> GPMPVFHTRTIESILEPVAQQISHLVIMHEEGEVDGKAIPDLTAPVAAVQAAVSNLVRVGKETVQTTEDQILKRDMPPAFIKVENACTKLVQAAQMLQSDP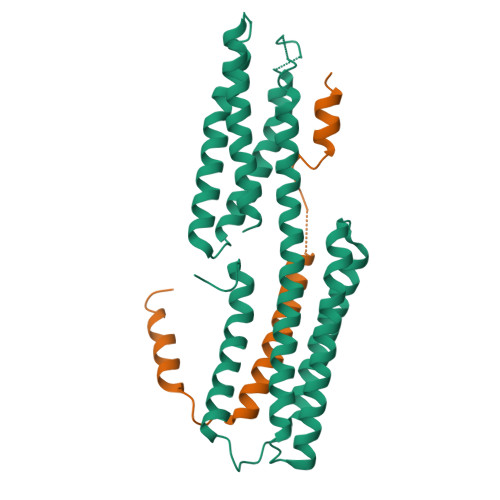YSVPARDYLIDGSRGILSGTSDLLLTFDEAEVRKIIRVCKGILEYLTVAEVVETMEDLVTYTKNLGPGMTKMAKMIDERQQELTHQEHRVMLVNSMNTVKELLPVLISAMKIFVTTKNSKNQGIEEALKNRNFTVEKMSAEINEIIRVLQL;> GPGELAYALNNFDKQIIVDPLSFSEERFRPSLEERLESIISGAALMADSSCTRDDRRERIVAECNAVRQALQDLLSEYMGNAGRKERSDALNSAIDKMTKKT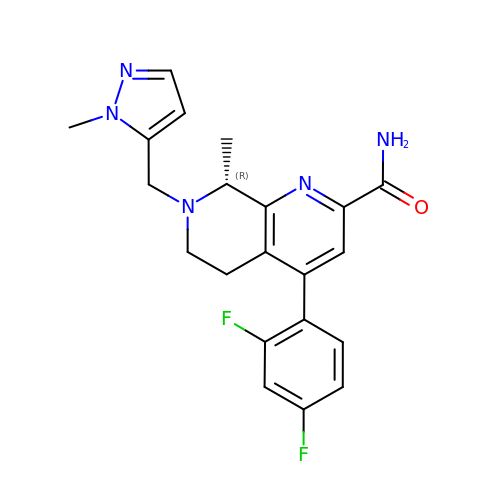(8~{R})-4-[2,4-bis(fluoranyl)phenyl]-8-methyl-7-[(2-methylpyrazol-3-yl)methyl]-6,8-dihydro-5~{H}-1,7-naphthyridine-2-carboxamide | C21 H21 F2 N5 O | JPQHCBORHNWOOF-GFCCVEGCSA-N>[2x]SHMAHQDALPRLPVPPLQQSLDYYLKALQPIVSEEEWAHTKQLVDEFQTSGGVGERLQKGLERRAKKMENWLSEWWLKTAYLQFRQPVVIYSSPGVILPKQDFVDLQGQLRFAAKLIEGVLDFKSMIDNETLPVEFLGGQPLCMNQYYQILSSCRVPGPKQDSVVNFLKSKRPPTHITVVHNYQFFELDVYHSDGTPLTSDQIFVQLEKIWNSSLQSNKEPVGILTSNHRNTWAKAYNNLIKDKVNRESVNSIQKSIFTVCLDKQVPRVSDDVYRNHVAGQMLHGGGSKFNSGNRWFDKTLQFIVAEDGSCGMVYEHAAAEGPPIVALVDHVMEYTKKPELVRSPMVPLPMPKKLRFNITPEIKNDIEKAKQNLSIMIQDLDIMMLTFHHFGKDFPKSEKLSPDAFIQVALQLAYYRIYGQACATYESASLRMFHLGRTDTIRSASIDSLAFVKGMGDSTVPEQQKVELLRKAVQAHRAYTD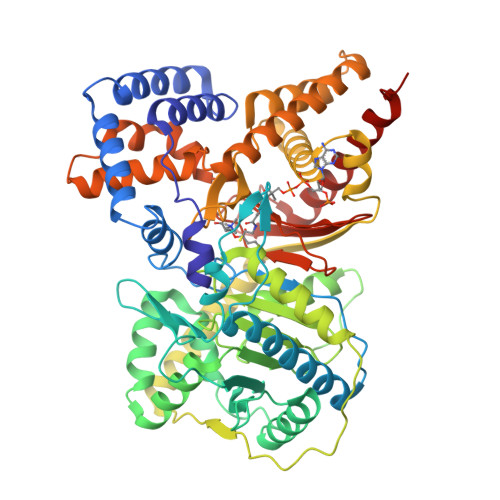RAIRGEAFDRHLLGLKLQAIEDLVSMPDIFMDTSYAIAMHFNLSTAQVPAKTDCVGFFGPVVPDGYGICYNPMEAHINFSVSAYNSCAETNAARMAHYLEKALLDMRTLLQNHPRAK3-(1,3,7-TRIHYDRO-9-D-RIBITYL-2,6,8-PURINETRIONE-7-YL) 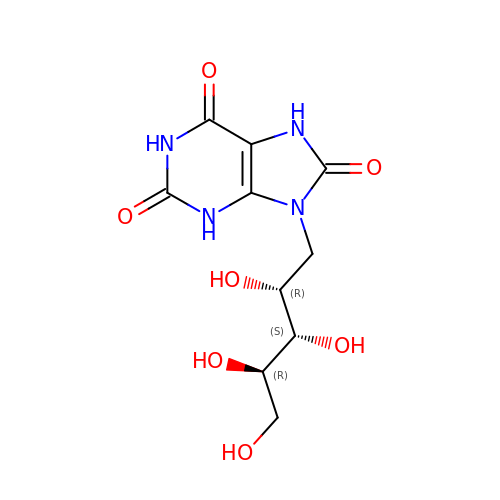| C10 H14 N4 O7 | XIBHHWBJHOTHGZ-KODRXGBYSA-N>MATHHTLWMGLALLGVLGDLQAAPEAQVSVQPNFQQDKFLGRWFSAGLASNSSWLREKKAALSMAKSVVAPATDGGLNLTSTFLRKNQCETRTMLLQPAGSLGSYSYRSPHFGSTYSVSVVETDYDQYA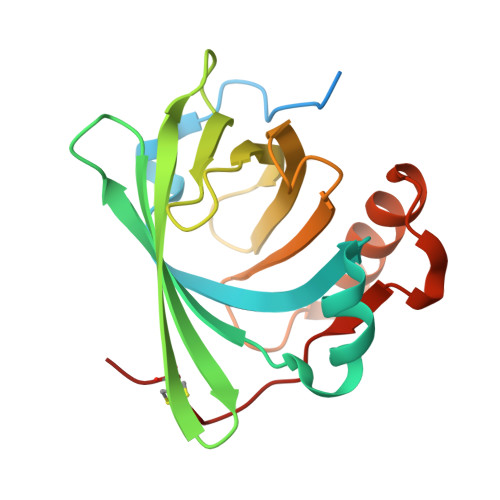LLYSQGSKGPGEDFRMATLYSRTQTPRAELKEKFTAFCKAQGFTEDTIVFLPQTDKCMTEQ[2x]> CNWTGVKCNRRGEVSEIQLKEKQLQGSLPVTSLRSLKSLTSLTLSSLQLTGVIPKEIGDFTELELLDLSDNSLSGDIPVEIFRLKKLKTLSLNTNNLEGHIPMEIGNLSGLVELMLFDNKLSGEIPRSIGELKNLQVLRAGGNKNLRGELPWEIGNCENLVMLGLAETSLSGKLPASIGNLKRVQTIAIYTSLLSGPIPDEIGYCTELQNLYLYQNSISGSIPTTIGGLKKLQSLLLWQNNLVGKIPTELGNCPELWLIDFSENLLTGTIPRSFGKLENLQELQLSVNQISGTIPEELTNCTKLTHLEIDNNLITGEIPSLMSNLRSLTMFFAWQNKLTGNIPQ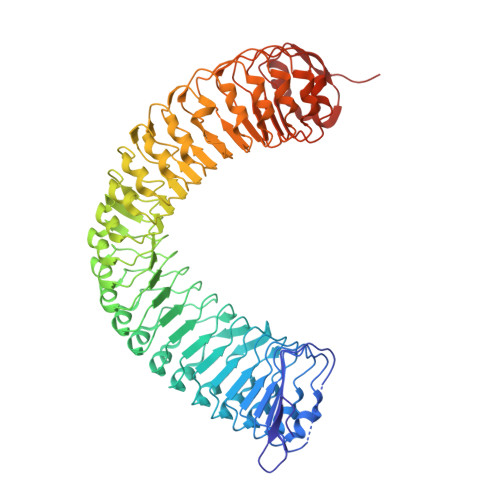SLSQCRELQAIDLSYNSLSGSIPKEIFGLRNLTKLLLLSNDLSGFIPPDIGNCTNLYRLRLNGNRLAGSIPSEIGNLKNLNFVDISENRLVGSIPPAISGCESLEFLDLHTNSLSGSLLGTTLPKSLKFIDFSDNALSSTLPPGIGLLTELTKLNLAKNRLSGEIPREISTCRSLQLLNLGENDFSGEIPDELGQIPSLAISLNLSCNRFVGEIPSRFSDLKNLGVLDVSHNQLTGNLNVLTDLQNLVSLNISYNDFSGDLPNTPFFRRLPLSDLASNRGLYISNAIST> GMSKGEGTIANHLLEQQIKAFPKVAQQYYPRELSILRLQDAMKFVKELFTVCETVLSLNALSRSTGVPPELHVLLPQISSMMKRKIVQDDILKLLTIWSDAYVVELNSRGELTMNLPKRDNLTTLTNKSRTLAFVERAESWYQQVIASKDEIMTDVPAFKINKRRSSSN

The process of eukaryotic DNA replication begins during G1 phase with the loading of the minichromosome maintenance (MCM) heterohexamer comprising Mcm2–7 subunits into head-to-head double hexamers with double-stranded DNA passing through the length of a long central channel. This topological loading requires the Origin Recognition Complex (ORC), Cdc6 and Cdt1 proteins. In budding yeast, Cdt1 forms a stable complex with MCM before loading. We propose that Cdt1 stabilizes a conformation of the MCM ring in which the Mcm2–5 gate is held open to allow duplex DNA passage required for helicase loading. To understand Cdt1–MCM at an atomic level, we determined crystal structures of two non-overlapping fragments of S. cerevisiae Cdt1 spanning amino acid residues 1–438 and 495–604.

The fragment comprises a pair of well-defined domains corresponding to the N domain (residues 14–298) and the M domain (residues 299–430). domain (WHD) family and is predictably similar to the geminin-binding M domain of mouse Cdt1. Further division of the C terminus of Cdt1 showed that fragments containing amino acid residues 271–496 and 495–604 interacted with both Mcm2 and 6, suggesting there are multiple interactions between Cdt1 and MCM subunits. By docking the crystal structure of NM Cdt1 into the Cdt1 density, an MCM interaction can be modelled, whereby the middle domain of Mcm2 is sandwiched between the A-domain and AAA+ domain of Mcm2 and extends to contact the A-domain of Mcm6, following the outer perimeter of the MCM N-terminal domain. In summary, Cdt1 makes extensive contacts with the outer perimeter of MCM, notably being sandwiched between the A and AAA+ domains of Mcm2.>MEVMNKENIIADAPSDVVKTVQQQVHLNQDEYKYLKQVEQILREGTRRDDRTGTGTISIFGMQSKYCLRNGTIPLLTTKRVYWKGVLEELLWFISGSTDGKLLMEKNVKIWEKNGDRAFLDNLGFTSREEGDLGPVYGFQWRHFGAKYVDCHTDYSGQGVDQLAEVIRQIKEQPDSRRIIMSAWNPSDLGQMVL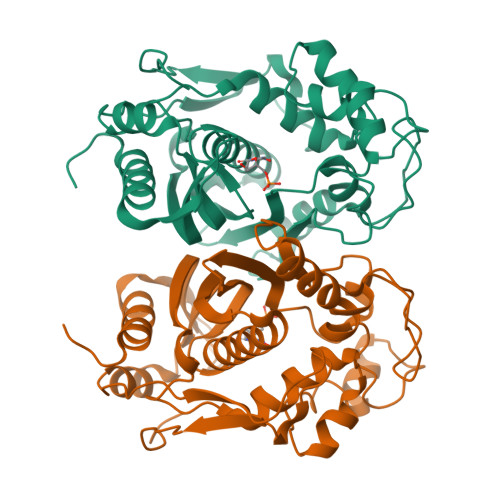PPCHTMCQFYVDNGELSCQLYQRSGDMGLGVPFNLASYGLLTHMIAKVCGLKPGTLVHTLGDAHVYSNHVDALKIQLDREPYAFPKIRFTRDVASIDDFTSDMIALDDYKCHPKIPMDMAV[2x]N-(4-{2-[(3-CHLOROBENZYL)AMINO]ETHYL}PHENYL)THIOPHENE-2-CARBOXIMIDAMIDE | C20 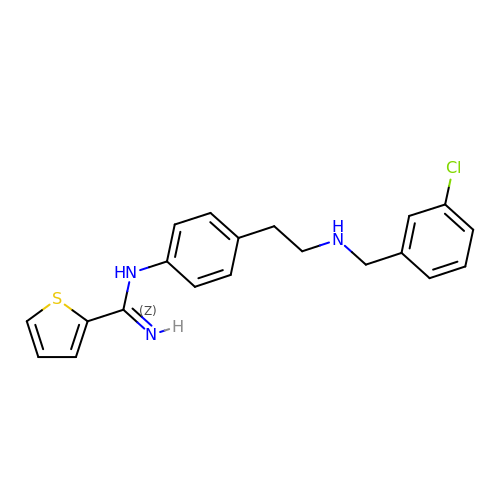H20 Cl N3 S | ZZVGLDBDDYESAB-UHFFFAOYSA-N>DAVIPPISCPENEEG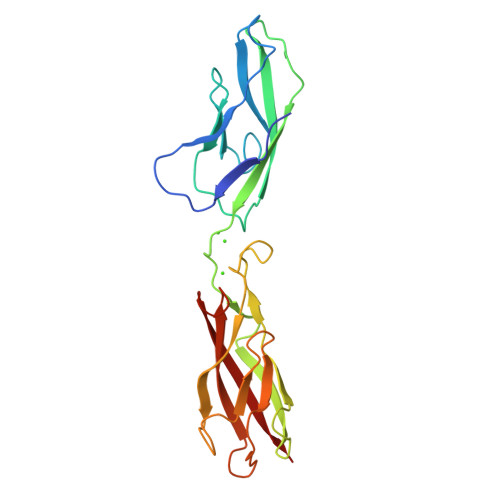EFPKNLVQIKSNRDKETKVFYSITGQGADKPPVGVFIIERETGWLKVTQPLDREAIAKYILYSHAVSSNGEAVEDPMEIVITVTDQNDNRPEFTQEVFEGSVAEGAVPGTSVMKVSATDADDDVNTYNAAIAYTIVSQDPELPHKNMFTVNRDTGVISVLTSGLDRESYPTYTLVVQAADLQGEGLSTTAKAVITVKD[2x]> GPGSHLAHPNLDTFTPEELLQQMKELLTENHQLKEAMKLNNQAMKGRFEELSAWTEKQKEERQ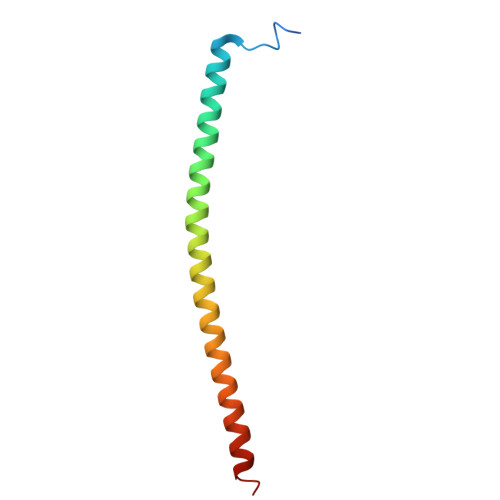FFEIQSKEAKERLMALSHE Among them, cyclic electron transfer around photosystem I (PSI CET) is an important mechanism that balances the ATP/NADPH ratio required for the Calvin–Benson cycle and reduces the ROS production. The NDH-1 complex is a key component of this pathway in most photosynthetic organisms and its inactivation leads to growth defects and even cell death under environmental stresses. Previous studies strongly suggest that, together with Fd, the NDH-1M module constitutes a key portion of the PSI CET pathway—electrons donated by photoreduced Fd are transferred to PQ via the chain of three conserved [4Fe-4S] clusters, corresponding to previously identified N6a, N6b, and N2 clusters in respiratory complex I19 (Fd-N6a-N6b-N2-PQ).

We purified the endogenous NDH-1L from the thermophilic cyanobacterium Thermosynechococcus elongatus BP-1 using a native polyhistidine tag on subunit NdhF1. Mass spectrometric analysis suggested that the amount of NdhV in the purified complex appeared to be substantially less than that of NdhS, which has a similar molecular weight as NdhV. This observation is in accordance with previous data that NdhV is a transiently associated subunit of NDH-121. We determined the cryo-EM structure of the NDH-1L complex at 3.6-Å resolution, which indeed lacks the NdhV subunit. Hereafter, we will refer to this complex as NDH-1LΔV. The first hint of the chemical identity of β-carotene was from the yellow color of the purified NDH-1LΔV complex revealed by the clear native-polyacrylamide gel electrophoresis (CN-PAGE) analysis. Absorption spectrum of the excised yellow band from the gel showed the characteristic absorption peaks of β-carotene, further confirming the presence of β-carotene in the purified NDH-1LΔV complex from T. elongatus thylakoid membranes. Given that we purified the endogenous NDH-1LΔV complex from T. elongatus thylakoid membranes with a mild detergent (digitonin), the lipids we found in the NDH-1L structure are very likely physiologically relevant and reflect their actual binding positions in NDH-1L in vivo, suggesting that lipids in NDH-1L may play important roles as lipids found in other photosynthesis complexes of cyanobacteria. To further examine the function of NdhV, we used the M55 (the ΔndhB strain of Synechocystis 6803) mutant thylakoid membranes that exhibit a complete loss of the Fd-dependent PQ reduction activity due to the lack of functional NDH-1 complexes. This activity can be partially restored when supplemented with purified T. elongatus NDH-1LΔV and can be further alleviated by addition of purified T. elongatus NdhV.

> MESGIDLQGQFISALQSLGLSHDLAKLLWLPLPMLMMLIVATVGVLVAVWLERKISAAVQQRIGPEYIGPLGILAPLADGLKLIFKEDVLPANSDRWLFTLGPAVVVIPVFLSYIIVPFGQNLLISNLAMGVFLWIALSSIAPIGLLMAGYASNNKYSLLGGLRAAAQSISYEIPLALAVLAVAMMSNGLGTVEIVEQQSQYGILSWNVWRQPIGFLVFWIAALAECERLPFDLPEAEEELVAGYQTEYAGMKFALFYLGAYVNLVLSALLVSVLYFGGWSFPIPLETIANLLGVSETNPFLQIAFAVLGITMTLIKAYFFVFLAILLRWTVPRVRIDQLLDLGWKFLLPVGLVNLLLTAGLKLAFPVAFGG;> MDLVTLAGQLNAGTILPETILIVTLLVVLLADLIQGRQADRWTPYFAIVGLGGAIATMIPLWTQPATISFFGSFISDHLSLFFRGLIALSALGTILMSIRYVEQTGSSLGEFMTILLTATVGGMFIAGAQELVFIFVALETLSIASYLLTGYTKRDSRSNEAALKYLLIGAASSAIFLYGSSLLYGLSGGHTQLPAIAQALSSESLGLVVALVFVIAGISFKISAVPFHQWTPDVYEGAPTPVVAFLSVGSKAAGFALAIRFLTLAFPSVTDQWQLIFTVLAILSMILGNVVALAQTSMKRMLAYSSIGQAGFVMIGFVVGTEAGYASMLFYLLVYLFMNLGAFTCVILFSLRTGTDQISEYAGLYQKDPLLTLGLSLCLLSLGGIPPLAGFFGKIYLFWAGWQAGAYGLVLLGLLTSVISIYYYIRVVKMMVVKEPQEMSEAVRNYPEVSWSSFGLRPLQVGLVMTVIATSLAGILANPLFNLVNTAVWDVPQLANQPTVMEVAYQALSPAGKS;> MVAIPRLRDTATVFVLSGYEYFLGFLIICSLVPVLALAASALLRPKSGRMIRLTTYESGMEPIGGAWIQFNVRYYMFALVFVIFDVETVFLYPWAVAFHQLGLLAFIEALIFIAILVVALVYAWRKRALEWS;> MSTFPWLTTIILFPIVAALAIPFIPDPTGKGRPIRWYALAVGLIDFALIVYAFTNFYDLNTPGMQLWESYDWIPEIGLRWSVGADGLSMPLILLTGFITTLAILAAWPVTLKPRLFYFLMLAMYGGQIAVFAVQDMLVFFLAWELELIPVYLLLAIWGGHKRQYAATKFILYTAGSSLFILVAGLAMAFYGDTVSFDMQTLAAKDYALGFQLLVYAGFLVAYGVKLPIVPLHTWLPDAHGEATAPVHMLLAGILLKMGGYALIRMNVDMLPAAHAKFAPVLVILGVVNIIYAALTSYAQRNLKRKIAYSSISHIGFVLIGIASFTNLGMSGAVLQMVSHGLIGASLFFLVGATYDRTHTLILEEMGGVGQKMKKIFAMFTACSLASLALPGMSGFVAELMVFIGFATSDAYSLPFRVIVVFLAAVGVILTPIYLLSMLREIFYGPENKELVEHEALVDAEPREVFIIACLLVPIIGIGLYPKLLTQIYDATTGQVIARAREVLPTLAQQTEQPLGILPMVAPQLKANAQ;> MQLTYVLILAALLFCIGIYGLVTSRNAVRVLMSIELLLNAVNLNLIGFANYLDGQQIKGQVFAVFVITVAAAEAAVGLAIILAIYRNRDTVDMEKFNLLKW;> MEPLYQYAWLIPVLPLLGALIVGFGLIAFSETTSKLRRPSAIFIMALMAIAMGHSLTLFWSQVQGHLPYTQMIEWAAAGNLHIAMGYVIDPLAALMLVIVTTVAFLVMLYSDGYMAHDPGYVRFFAYLSLFGSSMLGLVVSPNLVQVYIFWELVGMCSYLLIGFWYDRKSAAEAAQKAFVTNRVGDFGLLLGMVGLFWATGTFDFAGMGDRLTELVNTGLLSPSLAAILAILVFLGPVAKSAQFPLHVWLPDAMEGPTPISALIHAATMVAAGVFLIARMFPVFEQLPQVMTTIAWTGAFTAFMGATIAITQNDIKKSLAYSTISQLGYMVMGMGVGAYSAGLFHLMTHAYFKAMLFLGSGSVIHSMEGVVGHNPDLAQDMRYMGGLRKYMPITGATFLVGCLAISGVPPFAGFWSKDEILGAVFHANPAMWLLTWLTAGLTAFYMFRMYFMTFEGKFRNVPPERQEHHDHHSHHAAVPHESPWTMTLPLVVLAIPSTLIGFVGTPFNNLFEVFIHAPGEEKVAEHAVDLTEFLILGGSSVGIGLMGITVAYLMYLKGTPSPQAIAKAIQPLYQFSLHKWYFDELYEAVFIKGCRRLARQVLEVDYNVVDGVVNLTGFVTMVTGEGLKYLQNGRAQFYALIVLLAVLGFVIFSVQT;> MDLATLTQTITFFALAAAVIIAALGVVLLDNVVYSAFLLGGVFLSIAGLYILMNADFVSAAQILIYVGAVNVLILFAIMLVNKRETYTPVPGRWLRQGGAAVVSLGVFALLTKMILQTPWQLSSVPPTPDSITTIGQHFFSDFLLPFELASVLLLMALIGAVVLARRELVLEPEPILGEEVVPPLELPERPREPVALSEK;> MPKIETRTEPMVINMGPHHPSMHGVLRLMVTLDGEDVIDCEPVIGYLHRGMEKIAENRTNIMFIPYVSRWDYAAGMFNEAVTVNAPEKLAGIPVPKRASYIRVIMLELNRIANHLLWLGPFLADVGAQTPFFYIFREREYIYDLFEAATGMRFINNNYFRIGGVAADLTYGWVTKCRDFCDYFLPKVDEYERLITNNPIFVRRLQGVGKISREEAINWGLSGPMLRASGVKWDLRKVDHYECYDDFDWDVPVATEGDCLARYIVRIQEMRESVKIIRQALDGLPGGPYENLEAKRMLEGAKSEWNGFDYQYIGKKLSPTFKIPKGEHYVRVESGKGELGIYLIGDDNVFPWRWKIRPPDFNNLQVLPQLLKGMKVADIVAILGSIDVIMGSVDR;> MKFLNQITNYAKEAVQSAKYIGQGLSVTFDHMRRRPITVQYPYEKLIPSERFRGRIHFEFDKCIACEVCVRVCPINLPVVDWVFNKELKKKELKHYSIDFGVCIFCANCVEYCPTNCLSVTEEYELATYDRHELNYDSVAMGRIPYKVTQDPMVTPIREFAYLPAGVMSGHDLPAGAQRAGERPEAIANTAKSSEN;> MSDTPEAPIVEAGPVGRLLQSQNLSVESLGRDASGVEMIKVDRDRLLAVCQTLYADGFNYLRCQAAYDSGPGQDLVSTYHLIKLSDNADRPPEVRIKVFVPRDDPRVPSVYWIWKTADWQERESYDMFGIVYEGHPNLKRILMPEDWVGWPLRKDYITPDFYELQEAY;> MTNTTSPAILNPIARPEVPQELAENIILTSLNDVYDWARLSSLWPLMYGTACCFIEFAAMIGSRFDFDRFGLVPRNSPRQADLIITSGTITMKMAPALVRLYEQMPSPKYVIAMGACTITGGMFSSDSYSAVRGVDKLIPVDVYLPGCPPRPEAIMDAIVKLRKKIANEHINERGNLAQTHRLFTAKHKMKPVPPILTGQYLNAPSRQAPPPALAAAMGIAVPALGEAVSETTSVAE;> MAVSTELLVLGVYGALAGLYLLVVPAIVYAYLNARWYVASSFERAFMYFLVTFFFPGLLLLAPFINFRPQPRSLNS;> MLLKSTTRHVHIYAGHVVDGEVHPDTETLTLNVDPDNELEWNEAALAKVEAKFRELVANAAGEDLTEYNLRRIGSDLEHFIRSLLMQGEIGYNLNSRVRNYSLGIPRVNHS;> MGLLAGYQFVKDLESAGALALFVPPEGGFEGRYQRRLRSKGYTTLPMSAPGLGDLAAYLTQEHGIRPAHTGKEDIRVYFQPPLVTYHLENLPPNAKGLVLWLIDGKRLSKQEFAYLAQLTQTLPKFKVVVEVGGDRVVRWEPLADWVAAA;> MAIKKGDLVKVVAEKLANSLEALASDHRYPPYLFEGRGEVVDIRGDYAQIKFPVPTPTVWLRLDQLEVAQ;> MDAVISVKPILLAMTPVFILLCLFFGTRNGFYDTDQYHGNGSAH;> MATDFNRGIMKFDGADSPAMIAISAVLILGFIAGLIWWALHTAYA;> MIRPIADTYPLLPLSKAQMGQRQEIINSHKRLWDKTMATDLIMTILPGMTVKVTNPNDTYYQFQGIVQRITDGKVAVLFEGGNWDKLVTFQASELEPVVVTPKEKAKAKK>[2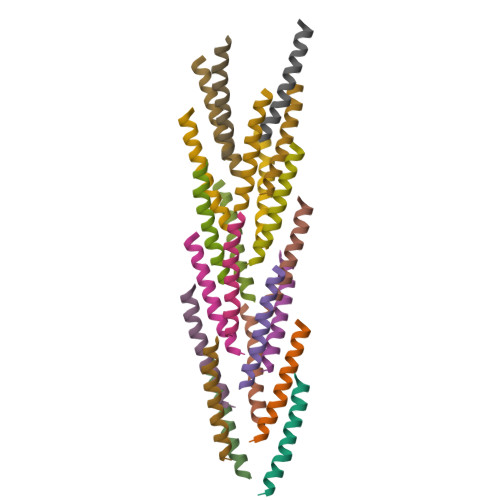1x]VSPVIATLLLILIAVAAAVLLYTWVS> GPMGKPARKGAEWKRFLKNNWVLLSTVAAVVLGITTGVLVREHSNLSTLEKFYFAFPGEILMRMLKLIILPLIISSMITGVAALDSNVSGKIGLRAVVY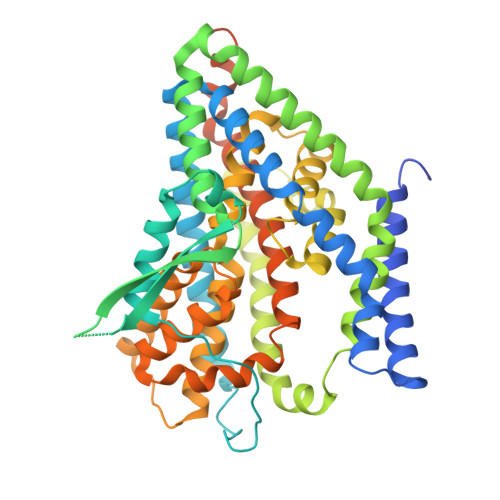YFATTLIAVILGIVLVVSIKPGVTQKVGEIARTGSTPEVSTVDAMLDLIRNMFPENLVQAAFQQYKTKREEVKPPSDPEMTMTEESFTAVMTTAISKTKTKEYKIVGMYSDGINVLGLIVFALVFGLVIGKMGEKGQILVDFFNALSDATMKIVQIIMWYMPLGILFLIAGCIIEVEDWEIFRKLGLYMATVLTGLAIHSIVILPLIYFIVVRKNPFRFAMGMAQALLTALMISSSSATLPVTFRCAEENNQVDKRITRFVLPVGATINMDGTALYEAVAAVFIAQLNDLDLGIGQIITISITATSASIGAAGVPQAGLVTMVIVLSAVGLPAEDVTLIIAVDCLLDRFRTMVNVLGDAFGTGIVEKLSKKELEQMDVSSEVNIVNPFALESTILDNEDSDTKKSYVNGGFAVDKSDTISFTQTSQF> ALQYKGVDWSSVMVEERAGVRYKNVNGQEKPLEYILAENGVNMVRQRVWVNPWDGNYNLDYNIQLARRAKAAGLGLYINFHYSDTWADPAHQTTPAGWPSDINNLAWKLYNYTLDSMNRFADAGIQVDIVSIGNEITQGLLWPLGKTNNWYNIARLLHSAAWGVKDSRLNPKPKIMVHLDNGWNWDTQNWWYTNVLSQGPFEMSDFDMMGVSFYPFYSASATLDSLRRSLNNMVSRWGKEVAVVETNWPTSCPYPRYQFPADVRNVPFSAAGQTQYIQSVANVVSSVSKGVGLFYWEPAWI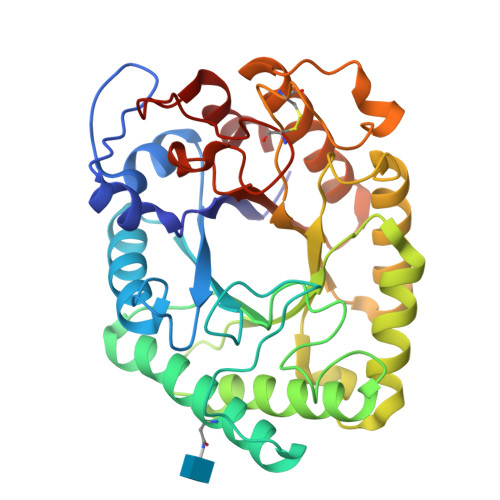HNANLGSSCADNTMFTPSGQALSSLSVFHRI> MSRKRSTKPKPAAKIALKKENDQFLEALKLYEGKQYKKSLKLLDAILKKDGSHVDSLALKGLDLYSVGEKDDAASYVANAIRKIEGASASPICCHVLGIYMRNTKEYKESIKWFTAALNNGSTNKQIYRDLATLQSQIGDFKSALVSRKKYWEAFLGYRANWTSLAVAQDVNGERQQAINTLSQFEKLAEGKISDSEKYEHSECLMYKNDVM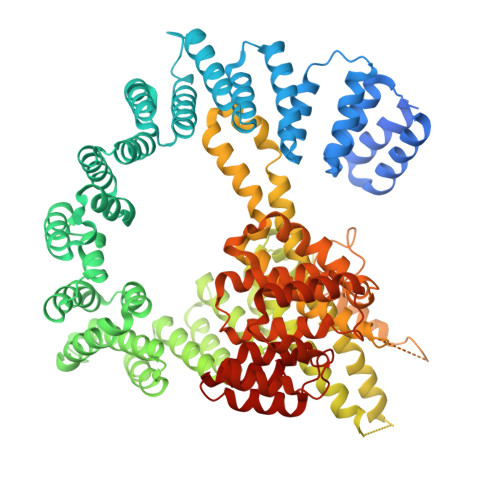YKAASDNQDKLQNVLKHLNDIEPCVFDKFGLLERKATIYMKLGQLKDASIVYRTLIKRNPDNFKYYKLLEVSLGIQGDNKLKKALYGKLEQFYPRCEPPKFIPLTFLQDKEELSKKLREYVLPQLKRGVPATFSNVKPLYQRRKSKVSPLLEKIVLDYLSGLDPTQDPIPFIWTNYYLSQHFLFLKDFPKAQEYIDAALDHTPTLVEFYILKARILKHLGLMDTAAGILEEGRQLDLQDRFINCKTVKYFLRANNIDKAVEVASLFTKNDDSVNGIKDLHLVEASWFIVEQAEAYYRLYLDRKKKLDDLESLKKEVESDKSEQIANDIKENQWLVRKYKGLALKRFNAIPKFYKQFEDDQLDFHSYCMRKGTPRAYLEMLEWGKALYTKPMYVRAMKEASKLYFQMHDDRLKRKSDSLDENSDEIQNNGQNSSSQKKKAKKEAAAMNKRKETEAKSVAAYPSDQDNDVFGEKLIETSTPMEDFATEFYNNYSMQVREDERDYILDFEFNYRIGKLALCFASLNKFAKRFGTTSGLFGSMAIVLLHATRNDTPFDPILKKVVTKSLEKEYSENFPLNEISNNSFDWLNFYQEKFGKNDINGLLFLYRYRDDVPIGSSNLKEMIISSLSPLEPHSQNEILQYYL> GSSSPPSPPLDLHVTDAGRKHIAIAWKPPEKNGGSPIIGYHVEMCPVGTEKWMRVNSRPIKDLKFKVEEGVVPDKEYVLRVRAVNAIGVSEPSEISENVVAKDPDCK

Titin is a protein expressed in the skeletal and cardiac, or striated, muscle of vertebrates that plays various roles in muscle structure and function. Encoded by the gene TTN, titin spans half a sarcomere (the basic contractile unit of muscle) and has various functions including preventing sarcomere over-extension (Gautel and Djinović-Carugo, 2016), acting as a molecular ruler for thick filament formation and as a hub for numerous signalling molecules (Kruger and Linke, 2011, Linke and Hamdani, 2014). Fn3 domains are only found in the A-band region of titin, where they are arranged with Ig domains in a pattern termed super-repeats, which themselves are repeated. Fn3 domains have a characteristic beta sandwich fold, with a core of hydrophobic residues as the “filling” between two beta sheets that pack against each other face-to-face.

Fn3-3 and Fn3-11 are found in the non-repetitive region of A-band titin near the tip of the thick filament, Fn3-20 is in the second D-zone super-repeat and Fn3-49, Fn3-56, Fn3-85 and Fn3-90 are located in the 1st, 2nd, 6th and 7th C-zone super-repeats, respectively. Structural predictions of the three variant domains suggest little change to the backbone trace of the proteins and that no clashes would be introduced upon mutation. All domains with variants from HCM patients were solubly expressed in bacteria (data not shown), however Fn3-11 Ala16872Pro was unfolded as evidenced by 1D NMR and its decrease in elution volume (and increased hydrodynamic radius) compared to WT in size exclusion chromatography. We also characterised the effects of three further rare missense variants found in patients with HCM: Fn3-11 Ala16872Pro renders its domain unfolded (contrary to the predicted domain structure) but is still solubly expressed in bacteria, whilst Fn3-85 Ser27083Pro and Fn3-90 Arg27839Gln do not affect the folding of their domain but reduce its thermal stability. The negative effects of Ala16872Pro on Fn3-11 are easier to rationalise as it renders the domain unfolded, though soluble. For two variants identified in congenital myopathy patients, we have previously shown that missense variants that render the domain misfolded and insoluble when expressed in bacteria also do the same when expressed in cardiac and skeletal cells, giving no reason to suggest expressing Fn3-11Ala16872Pro in mammalian cells would “rescue” folding of the domain via chaperone-mediated folding.>[4x]FTCPECRPELCGDPGYCEYGTTKDACDCCPVCFQG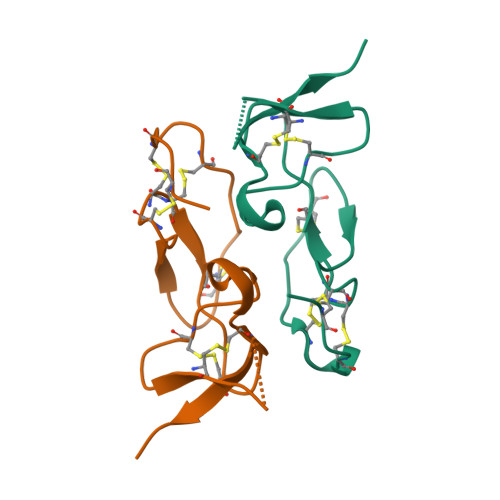PGGYCGGPEDVFGICADGFACVPLVGERDSQDPEIVGTCVKIP> MNTYFDIPHRLVGKALYESYYDHFGQMDILSDGSLYLIYRRATEHVGGSDGRVVFSKLEGGIWSAPTIVAQAGGQDFRDVAGGTMPSGRIVAASTVYETGEVKVYVSDDSGVTWVHKFTLARGGADYNFAHGKSFQVGARYVIPLYAATGVNYELKWLESSDGGETWGEGSTIYSGNTPYNETSYLPVGDGVILAVARVGSGAGGALRQFISLDDGGTWTDQGNVTAQNGDSTDILVAPSLSYIYSEGGTPHVVLLYTNRTTHFCYYRTILLAKAVAGSSGWTERVPVYSAPAASGYTSQVVLGGRRILGNLFRETSSTTSGAYQFEVYLGGVPDFESDWFSVSSNSLYTLSHGLQRSPRRVVVEFARSSSPSTWNIVMPSYFN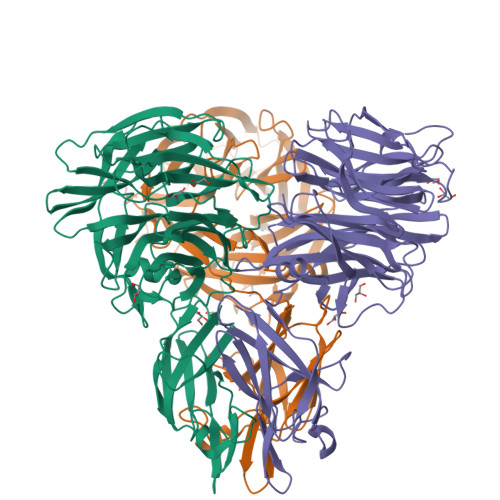DGGHKGSGAQVEVGSLNIRLGTGAAVWGTGYFGGIDNSATTRFATGYYRVRAWI> VKNPSLICAPVMADSIDKMVIETSKAHELGADLVEIRLDWLKDFNPLEDLKTIIKKSPLPTLFTYRPKWEGGQYEGDENERRDVLRLAMELGADYIDVELQVASEFIKSIDGKKPGKFKVIVSSHNYQNTPSVEDLDGLVARIQQTGADIVKIATTAVDIADVARMFHITSKAQVPTIGLVMGERGLMSRILCSKFGGYLTFGTLDSSKVSAPGQPTIKDLLDLYNFRRIGPDTKVYGIIGKPVSHSKSPIVHNQAFKSVDFNGVYVHLLVDNLVSFLQAYSSSDFAGFSCTIPHKEAALQCCDEVDPLAKSIGAVNTILRRKSD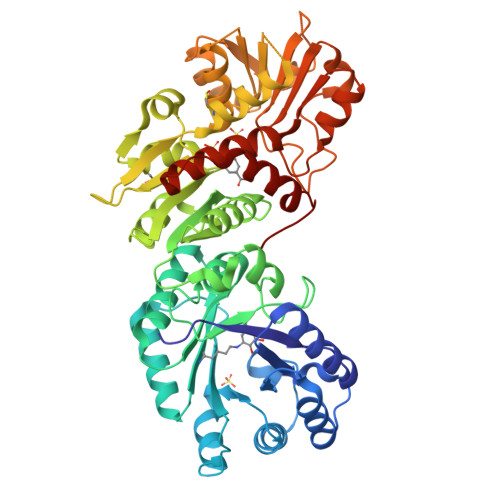GKLLGYNTDCIGSISAIEDGLRSSGDPSSVPSSSSPLASKTVVVIGAGGAGKALAYGAKEKGAKVVIANRTYERALELAEAIGGKALSLTDLDNYHPEDGMVLANTTSMGMQPNVEETPISKDALKHYALVFDAVYTPRITRLLREAEESGAITVSGSEMFVRQAYEQFEIFTGLPAPKELYWQIMSKYGSRENLYFQ>GPGSMDGSDGARRVLVINSGSSSLKFQLVDPEFGVAASTGIVERIGEESSPVPDHDAALRRAFDMLAGDGVDLNTAGLVAVGHRVVHGGNTFYRPTVLDDAVIARLHELSELAPLHNPPALQGIEVARRLLPDIAHVAVFDTGFFHDLPPAAATYAIDRELADRWQIRRYGFHGTSHRYVSEQAAAFLDRPLRGLKQIVLHLGNGCSASAIAGTRPLDTSMGLTPLEGLVMGTRSGDIDPSIVSYLCHTAGMGVDDVESMLNHRSGVVGLSGVRDFRRLRELIESGDGAAQLAYSVFTHRLRK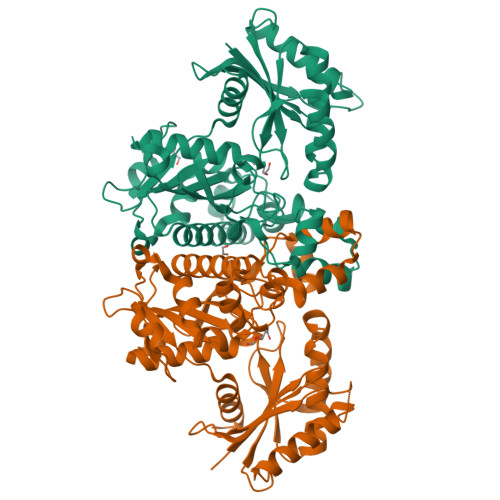YIGAYLAVLGHTDVISFTAGIGENDAAVRRDAVSGMEELGIVLDERRNLAGGKGARQISADDSPITVLVVPTNEELAIARDCVRVLGG[2x]>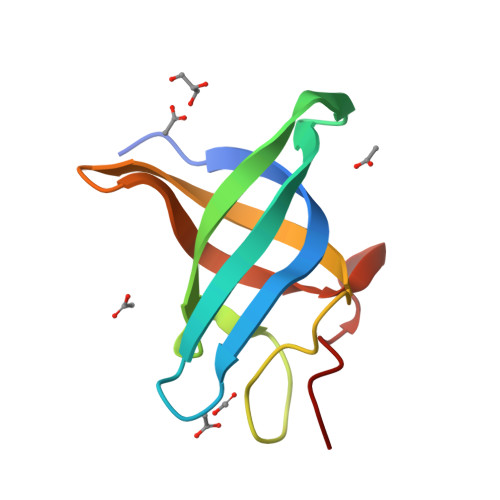[2x]GSDPQVLRGSGHCKWFNVRMGFGFISMTSREGSPLENPVDVFVHQSKLYMEGFRSLKEGEPVEFTFKKSSKGFESLRVTGPGGNPCLGNE> MDPDQYSIEADKKFKYSAKLSDYPTLQDAASAAVDGLLIDRDYNFYGGETVDFGGKVLTIECKAKFIGDGNLIFTKLGKGSRIAGVFMESTTTPWVIKPWTDDNQWLTDAAAVVATLKQSKTDGYQPTVSDYVKFPGIETL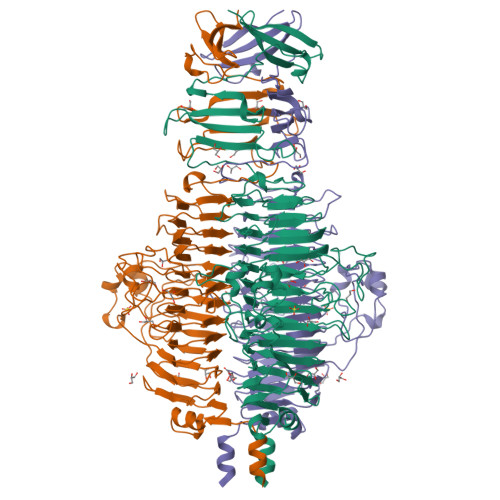LPPNAKGQNITSTLEIRECIGVEVHRASGLMAGFLFRGCHFCKMVDANNPSGGKDGIITFENLSGDWGKGNYVIGGRTSYGSVSSAQFLRNNGGFERDGGVIGFTSYRAGESGVKTWQGTVGSTTSRNYNLQFRDSVVIYPVWDGFDLGADTDMNPELDRPGDYPITQYPLHQLPLNHLIDNLLVRGALGVGFGMDGKGMYVSNITVEDCAGSGAYLLTHESVFTNIAIIDTNTKDFQANQIYISGACRVNGLRLIGIRSTDGQSLTIDAPNSTVSGITGMVDPSRINVANLAEEGLGNIRANSFGYDSAAIKLRIHKLSKTLDSGALYSHINGGAGSGSAYTQLTAISGSTPDAVSLKVNHKDCRGAEIPFVPDIASDDFIKDSSCFLPYWENNSTSLKALVKKPNGELVRLTLATL> MVMGIFANCIFCLKVKYLPQQQKKKLQTDIKENG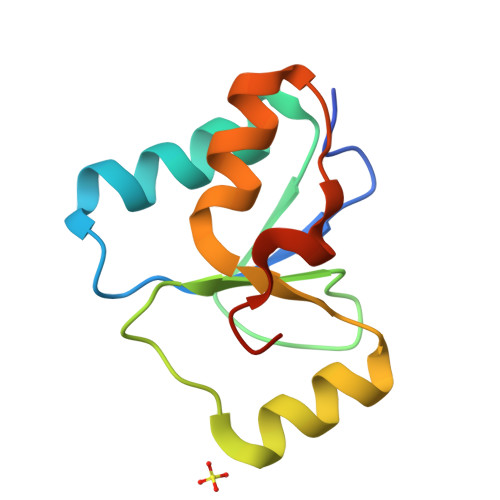GKFSASLNPQCTHIILDNADVLSQYQLNSIQKNHVHIANPDFIWKSIREKRLLDVKNYDPYKPLDI>NNLISFTMKRIVLFLILLTKAASANLISFTFKKFNETNLILQRDATVSSGKLRITKAAENGVPTAGSLGRAFYSTPIQIWDNTTGTVASWATSFTFNLQAPNAASPADGLAFALVPVGSQPKDKGGFLGLFDSKNYASSNQTVAVEFDTFYNGGWDPTERHIGIDVNSIKSIKTTSWDFANGENAEVLITYDSSTNLLVASL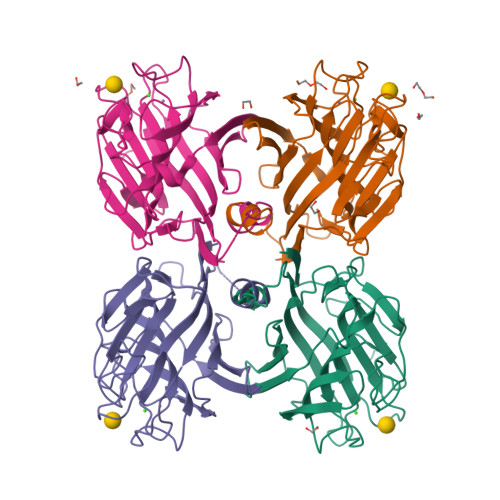VHPSQKTSFIVSERVDLTSVLPEWVSVGFSATTGLSKGYVETNEVLSWSFASKLSINKEDEENKLAIFNLEGKAINNLA[4x]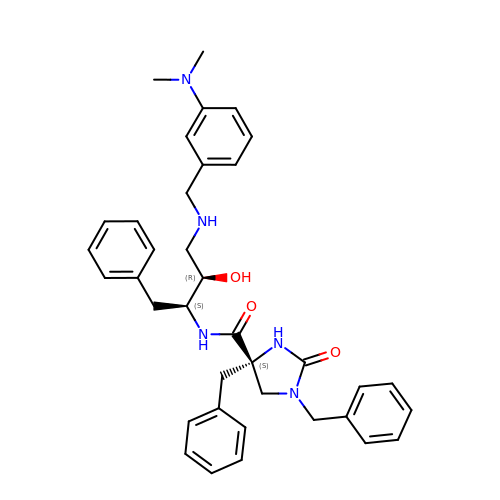(4S)-1,4-dibenzyl-N-[(1S,2R)-1-benzyl-3-{[3-(dimethylamino)benzyl]amino}-2-hydroxypropyl]-2-oxoimidazolidine-4-carboxamide | C37 H43 N5 O3 | DCJGHBWTJFHQCR-UEHMVRIRSA-N> SNTGEPAPVLSSPPPADVSTFLAFPSPEKLLRLGPKSSVLIAQQTDTSDPEKVVSAFLKVSSVFKDEATVRMAVQDAVDALMQKAFNSSSFNSNTFLTRLLVHMGLLKSEDKVKAIANLYGPLMALNHMVQQDYFPKALAPLLLAFVTKPNSALESCSFAR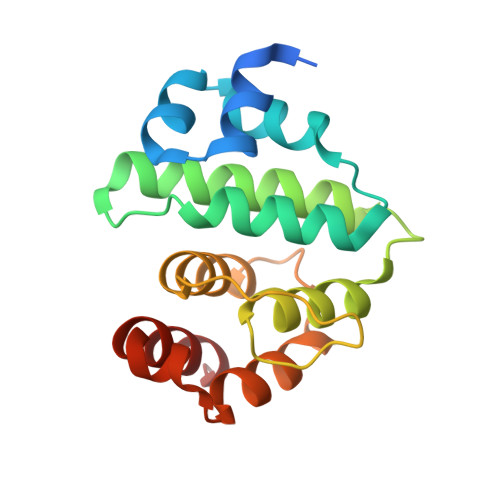HSLLQTLYKV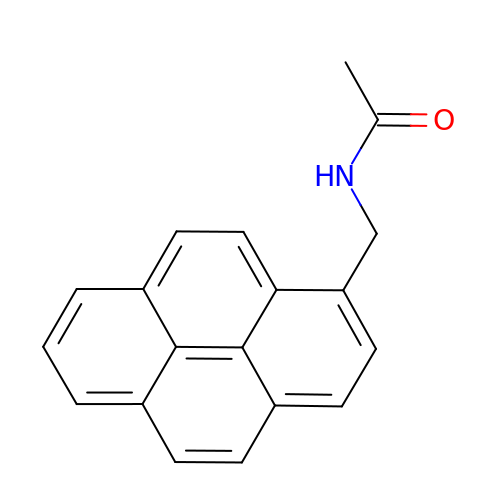N-(pyren-1-ylmethyl)acetamide | C19 H15 N O | IGDIETIXWIPXQF-UHFFFAOYSA-N> AKRQWALEDFEIGRPLGKGKFGNVYLAREKQSKFILALKVL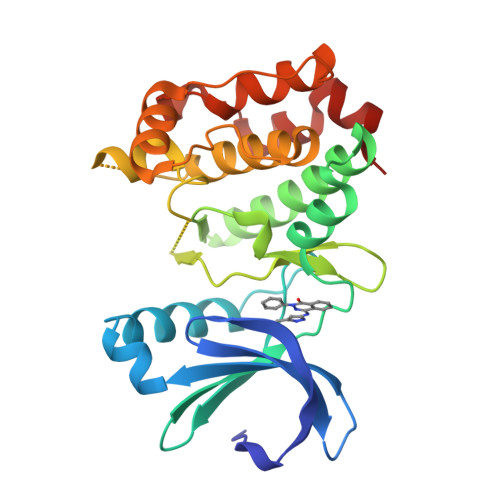FKAQLEKAGVEHQLRREVEIQSHLRHPNILRLYGYFHDATRVYLILEYAPLGTVYRELQKLSKFDEQRTATYITELANALSYCHSKRVIHRDIKPENLLLGSAGELKIADFGWSVHAPSSRRAALCGTLDYLPPEMIEGRMHDEKVDLWSLGVLCYEFLVGKPPFEANTYQETYKRISRVEFTFPDFVTEGARDLISRLLKHNPSQRPMLREVLEHPWITANSSKPS>[11x]SGRPMDKCWFTLDNAHYPPPSLDSMRSGHPISPASLGHLIPSLAHLDQIINAKAIEPFPATMDIHGPTIIEDFKWDHSHEYSLSLGGKVPIPLAPAGVPFVDLNVGLGGAFSRSVANYWEFDRLERYIMQPTRSYVQKCIER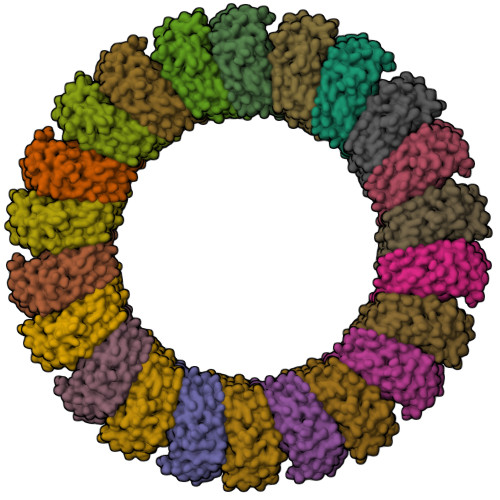DEVKRWIAKNKSMMMMGRWEVYMITGIIVARGGGRKKKEKTTGKEFSVEVTVEVPLIVEAGPGGKRNTARQKTWGTSQTGDFVWAVRLAKITKSGLHSDWKMETVFGKTSSFRGQKAIF;>[11x]SGRPMDNEEWFPLKQTHYPPPTIPSMKTGHPTGPISIGHIIPDLRHLDNVINCKGFEPFPPNMDVFTAHYEQCHFGDHLNSEFVVQAKAAAPIENIVPGVDVTGSAGLHHTNITSDRWEYDSVVEYAVYPTRQYIDRLLESKEVRQYIQKSKKLLGGWCVYMVTGIMVARGGGRNVTSEEKGAGVSGNVGFQVPGIGEFAPEVGWDTKTKTKVNAHHTTDFVCAIRLVKIAKSGLRSSWTMKKVTREF5-fluoro-3-phenyl-2-[(1S)-1-(7H-purin-6-ylamino)propyl]quinazolin-4(3H)-one 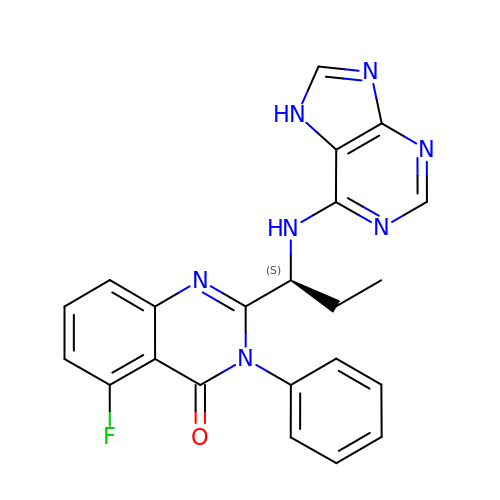| C22 H18 F N7 O | IFSDAJWBUCMOAH-HNNXBMFYSA-N6-{[(3R,4R)-4-{[5-(3-fluorophenyl)pentyl]oxy}pyrrolidin-3-yl]methyl}-4-methylpyridin-2-amine 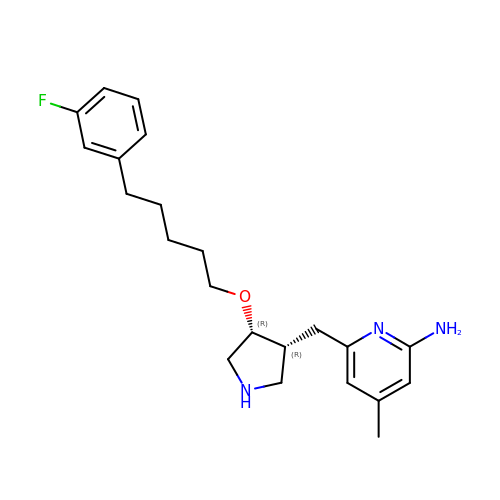| C22 H30 F N3 O | AQTALODLFZOZJL-NQIIRXRSSA-N>MNDFHRDTWAEVDLDAIYDNVENLRRLLPDDTHIMAVVKANAYGHGDVQVARTALEAGASRLAVAFLDEALALREKGIEAPILVLGASRPADAALAAQQRIALTVFRSDWLEEASALYSGPFPIHFHLKMDTGMGRLGVKDEEETKRIVALIERHPHFVLEGLYTHFATADEVNTDYFSYQYTRFLHMLEWLPSRPPLVHCANSAASLRFPDRTFNMVRFGIAMYGLAPSPGIKPLLPYPLKEAFSLHSRLVHVKKLQPGEKVSFGATYTAQTEEWIGTIPIGYADGWLRRLQHFHVLVDGQKAPIV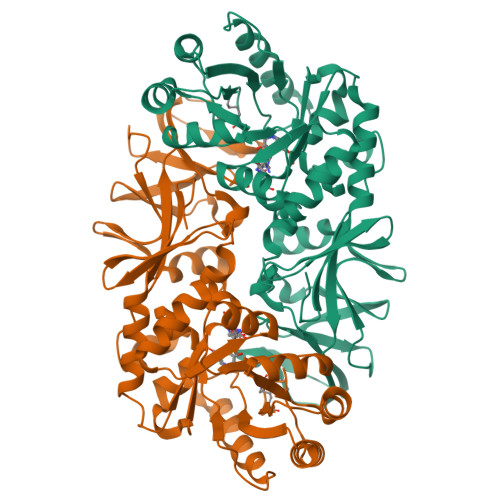GRICMDQCMIRLPGPLPVGTKVTLIGRQGDEVISIDDVARHLETINYEVPCTISYRVPRIFFRHKRIMEVRNAIGRGESSA[2x]Among them, Oligoribonuclease (Orn) is unique as its activity is required for clearing short RNA fragments, which is important for cellular fitness. Here, we show that Orn exhibits exquisite substrate preference for diribonucleotides. While other cellular RNases process oligoribonucleotides down to diribonucleotide entities, Orn is the one and only diribonucleotidase that completes the terminal step of RNA degradation. From this we propose a general model of RNA degradation, wherein a combination of exoribonucleases process oligoribonucleotides down to diribonucleotides and Orn completes RNA recycling by cleaving diribonucleotides to nucleoside monophosphates.

(A) Crystal structures of REXO2 bound to pApA and pApG. The structural overview (left) shows a C-terminal helix that is unique to Orn orthologs in higher eukaryotes and in the current crystal forms is stabilized by crystal packing contacts. Residue numbering for REXO2 refers to its cytosolic isoform lacking the mitochondria-targeting pre-sequence. Structures of OrnVc (and REXO2) with different diribonucleotides, including di-purine, di-pyrimidine and mixed substrates, revealed identical binding poses. Additional hydrogen bonding between purine residues and Orn in the 3' or 5' position correlates with a small, but detectable preference of OrnVc for purine-containing substrates. Together, the structural analysis uncovered Orn’s mode of substrate binding, which is conserved from bacteria to humans and indicates a unique selection for linear diribonucleotides with a 5’ phosphate.

>[2x]MAAGESMAQRMVWVDLEMTGLDIEKDQIIEMACLITDSDLNILAEGPNLIIKQPDELLDSMSDWCKEHHGKSGLTKAVKESTITLQQAEYEFLSFVRQQTPPGLCPLAGNSVHEDKKFLDKYMPQFMKHLHYRIIDVSTVKELCRRWYPEEYEFAPKKAASHRALDDISESIKELQFYRNNIFKKKIDEKKRKIIENGENEKTVS>[2x]MFTTRPTLQGTFGMVSSTHWLASQSAMAVLEDGGNAYDAAVAGAFVLHVVEPHLNGPAGEVPILLAPAGGEVRVLCGQGVAPAGATVAHYKGLGLDLVPGTGPLAAAVPGAFDAWMLLLRDHGTKPLADVLKYAVGYAEHGHAPVENVGVTVETVRELFETEWT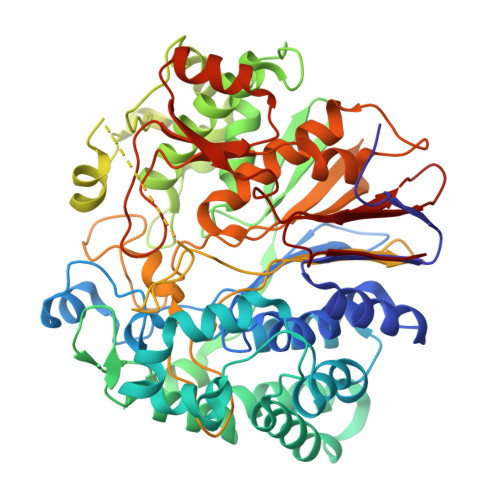TSADVYLPGGKAPRPGELLRNPTLAATWKRLLAEVAGAGDREAQIEAAREVWRTGFIAEALVRQARRPTMDTSGERHTGTLTAADLAGWSATYEAPATYDWNGWTVCKAGPWSQGPVLLQQLALLPPELPEYGSADYVHLLVEGCKLAMADREAWYGDAAEVPLDELLSAEYNAGRRELVGDKASHELRPGSPGGRTARLSAHADLVATGEPGFDPLGAGEPTAAMGAGEPTVAKLPASPVPGEPDVAADGSTRGDACHLDVVDRWGNMVAATPSGGWLQSNPVVPELGFPLGTRLQMTWLEEGLPNSLTPGRRPRTTLTPSIALRDGIPVMAFGTPGGDQQDQWQLHFFLAVALRARVRGGLDLQGAIDAPNWHNDSFPGSFYPRGMRPGSVTVEARMDPGIAAELRRRGHEVTVGPPWSEGRLCAVARDPRTGILSAAANPRGMQGYAVGR> ELTPDQQTLLHFIMDSYNKQRMPQEITNKILKEEFSAE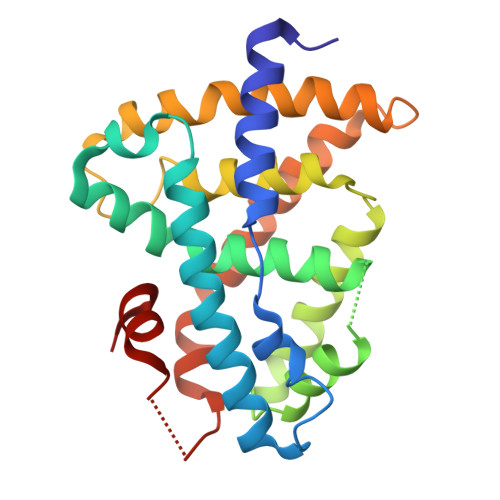ENFLILTEMATNHVQVLVEFTKKLPGFQTLDHEDQIALLKGSAVEAMFLRSAEIFNKKLPSGHSDLLEERIRNSGISDEYITPMFSFYKSIGELKMTQEEYALLTAIVILSPDRQYIKDREAVEKLQEPLLDVLQKLCKIHQPENPQHFAELLGRLTELRTFNHHHAEMLMSWRVNDHKFTPLLEEIWDVQ Of the known factors that promote muscle development, TRIM32 is an intriguing candidate for coordinating metabolism with cell growth. This protein is a member of the Tripartite motif (TRIM)-containing family of proteins defined by an N-terminal RING domain, one or two B-boxes, a coiled-coil domain, and a variable C-terminal region. In TRIM32, six Ncl-1, HT2A, Lin-41 (NHL) repeats comprise the C-terminus and are proposed to mediate the diverse functions of TRIM32, including cell proliferation, neuronal differentiation, muscle physiology and regeneration, and tumorigenesis. A single mutation in the B-box region of TRIM32 causes the multisystemic disorder Bardet-Biedl syndrome (BBS), while multiple mutations that cluster in the NHL domains result in the muscle disorders Limb-girdle muscular dystrophy type 2H (LGMD2H) and Sarcotubular Myopathy (STM). Our data show that TRIM32 promotes glucose metabolism through the stabilization of glycolytic enzyme levels.

Causative mutations in human LGMD2H cluster in the NHL repeats (Borg et al., 2009; Cossée et al., 2009; Frosk et al., 2005; Lazzari et al., 2019; Nectoux et al., 2015; Neri et al., 2013; Schoser et al., 2005), suggesting that this region may mediate protein-protein interactions important in disease prevention. We previously showed that mutations in Drosophila TRIM32 also show progressive larval muscle degeneration, despite modest sequence identity (~42%) across the NHL domains. To gain molecular-level insight into the functional conservation between the NHL regions in fly and mammalian TRIM32, we obtained a crystal structure of TRIM32_NHL at 2.6 Å resolution (Rwork/Rfree = 18.2/22.8%) (Figure 1—source data 1). We then used the TRIM32_NHL structure to construct a model for mouse TRIM32_NHL using SWISS-MODEL. Indeed, the superimposition of these two structures demonstrate that the NHL region of Drosophila TRIM32 is a faithful model to understand NHL function. Briefly, the C-terminal region of Drosophila TRIM32 containing all six NHL domains (AA 1061–1353) was fused in-frame with an N-terminal Glutathione S-transferase (GST) tag. To this end, we expressed and purified His-tagged Aldolase (Ald) or His-tagged Phosphoglycerate mutase 78 (Pglym), both of which were low or absent in control pulldowns. Both Ald and Pglym were found to directly interact with the NHL domains of TRIM32. Collectively, these data demonstrate that Ald and Pglym interact with the NHL domain of TRIM32 and in vivo, a subpopulation of these post-translationally modified glycolytic enzymes can be found in a complex with TRIM32. Another possibility, which we favor, is that the NHL domain of TRIM32 serves as a scaffold for the subcellular localization of glycolytic proteins to limit diffusion of substrates during glycolysis.

> GSTVAAAVAAAGITGAAGTIPKQVYLRKRQQLFQLGGRGSEPGSFTWPRGLAVGPDNSIVVADSSNHRVQVFDSNGIFVKEFGEYGNGEGEFDCLAGVAVNRIGQYIIADRYNHRIQVLDPQGRFLRAFGSQGTADGKFNYPWGVTTDALGFIYVCDKENHRVQVFQSDGSFVGKFGSCGRGEGQLEHPHYIAVSNTNRVIVSDSNNHRIQIFDVNGKVLSTVGGEGSDDGQFKFPRGVAVDDQGYIFVADSGNNRIQIFNPDGSFLKTFGSWGSGDSEFKGLEGVAIMSNGNILVCDRENHRVQVF Light absorption by rhodopsin induces isomerization of a single double bond of the retinal’s polyene chain, which triggers structural changes in the protein moiety to perform vital biological functions. Previous studies have suggested it is likely that GR could support ATP synthesis and compensate the poor energy production when the chlorophyll-dependent photosynthesis is low. Interestingly, GR has carotenoid binding capability similar to that found for xanthorhodopsin (XR). In this study, we present the X-ray crystal structure of GR and discuss the structural features that characterize the XR-like protein subgroup, to which it belongs.

The structure was determined to 2.0 Å resolution. Similar to other microbial rhodopsins, the seven transmembrane helices are bundled in a clockwise fashion when observed from the cytoplasmic side, and the all-trans-retinal chromophore is covalently bound to the opsin protein moiety via a Schiff base linkage with the Lys257 side chain. On the extracellular side, the B-C loop connecting helices B and C has a distinct antiparallel β-sheet structure similar to most microbial rhodopsins. However, unlike BR which has the β-sheet oriented towards the middle of its 7-TM helical bundle, the β-sheet of GR orients oppositely towards helices A and B. As a result, the tip of the B-C loop is facing towards the periphery of the GR molecule and the central ion-releasing cavity at the extracellular surface is exposed. When compared with the XR structure (shown in white), helices A, E, and G are slightly tilted inward towards the center of the helical bundle, resulting in a ~6.6 Å closer positioning of extracellular ends of helices E and G, whereas no obvious displacements are observed on the cytoplasmic side. Since GR in our crystals does not have any additional carotenoids, the movement of the extracellular end of helix E is likely to reflect the carotenoid-free structure of GR. First, there is a conserved Glu-Arg pair (Glu166-Arg174 in GR, Glu141-Arg152 in XR) on the extracellular side of helices D and E that can electrostatically interact to modulate the relative position of these helices. In addition, another conserved tyrosine residue on helix G of GR (Tyr249) participates in this interaction by forming a hydrogen bonded network with Glu166, whereas the corresponding tyrosine residues of XR and TR do not. Next, on the extracellular side of the Schiff base of GR, only one water molecule (wat-402 in XR) is mediating the hydrogen-bonded network among Asp121, Asp253 and retinal Schiff base, whereas BR has a water triad (wat-401, 402 and 406) among the corresponding Asp85, Asp212 and the Schiff base. In addition, similar to XR, GR also has the Asp121-His87 pair as the counterion (Asp85 in BR) of the Schiff base, confirming it is a conserved feature in XR-type proton pumps (XR/GR/TR) as well as proteorhodopsins (BPR/green-absorbing proteorhodopsin, GPR/Exiguobacterium sibiricum rhodopsin, ESR).

> MLMTVFSSAPELALLGSTFAQVDPSNLSVSDSLTYGQFNLVYNAFSFAIAAMFASALFFFSAQALVGQRYRLALLVSAIVVSIAGYHYFRIFNSWDAAYVLENGVYSLTSEKFNDAYRYVDWLLTVPLLLVETVAVLTLPAKEARPLLIKLTVASVLMIATGYPGEISDDITTRIIWGTVSTIPFAYILYVLWVELSRSLVRQPAAVQTLVRNMRWLLLLSWGVYPIAYLLPMLGVSGTSAAVGVQVGYTIADVLAKPVFGLLVFAIALVKTKADQESSEPHAAIGAAANKSGGSLIS>[8x]MPKRHREHIRKNLNILVEWTNYERLAMECVQQGILTVQMLRNTQDLNGKPFNMDEKDVRVEQHRRLLLKITQRGPTAYNLLINALRNINCLDAAVLLESVDE;>[8x]YQYKDILSVFEDAF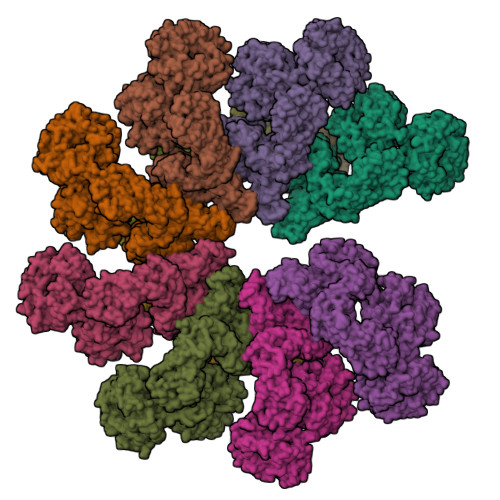VDNFDCKDVQDMPKSILSKEEIDHIIMSKDAVSGTLRLFWTLLSKQEEMVQKFVEEVLRINYKFLMSPIKTEQRQPSMMTRMYIEQRDRLYNDNQVFAKYNVSRLQPYLKLRQALLELRPAKNVLIDGVLGSGKTWVALDVCLSYKVQCKMDFKIFWLNLKNCNSPETVLEMLQKLLYQIDPNWTSRSDHSSNIKLRIHSIQAELRRLLKSKPYENCLLVLLNVQNAKAWNAFNLSCKILLTTRFKQVTDFLSAATTTHISLDHHSMTLTPDEVKSLLLKYLDCRPQDLPREVLTTNPRRLSIIAESIRDGLATWDNWKHVNCDKLTTIIESSLNVLEPAEYRKMFDRLSVFPPSAHIPTILLSLIWFDVIKSDVMVVVNKLHKYSLVEKQPKESTISIPSIYLELKVKLENEYALHRSIVDHYNIPKTFDSDDLIPPYLDQYFYSHIGHHLKNIEHPERMTLFRMVFLDFRFLEQKIRHDSTAWNASGSILNTLQQLKFYKPYICDNDPKYERLVNAILDFLPKIEENLICSKYTDLLRIALMAEDEAIFEEAHKQVQRFDDRVWFTNHGRFHQHRQIINLGDNEGRHAVYLHNDFCLIALASGQILLTDVSLEGEDTYLLRDESDSSDILRMAVFNQQKHLITLHCNGSVKLWSLWPDCPGRRHSGGSKQQLVNSVVKRFIGSYANLKIVAFYLNEDAGLPEANIQLHVAFINGDVSILNWDEQDQEFKLSHVPVLKTMQSGIRCFVQVLKRYYVVCTSNCTLTVWDLTNGSSNTLELHVFNVENDTPLALDVFDERSKTATVLLIFKYSVWRLNFLPGLSVSLQSEAVQLPEGSFITCGKRSTDGRYLLLGTSEGLIVYDLKISDPVLRSNVSEHIECVDIYELFDPVYKYIVLCGAKGKQVVHVHTLRSVSGSNSHQNREIAWVHSADEISVMTKACLEPNVYLRSLMDMTRERTQLLAVDSKERIHLIKPAISRISEWSTITPTHAASNCKINAISAFNDEQIFVGYVDGVIIDVIHDTALPQQFIEEPIDYLKQVSPNILVASAHSAQKTVIFQLEKIDPLQPNDQWPLMMDVSTKYASLQEGQYIILFSDHGVCHLDIANPSAFVKPKDSEEYIVGFDLKNSLLFLAYENNIIDVFRLIFSCNQLRYEQICEEEIAQKAKISYLVATDDGTMLAMGFENGTLELFAVENRKVQLIYSIEEVHEHCIRQLLFSPCKL BIS-(9-OCTYLAMINO(2-DIMETHYLAMINOETHYL)ACRIDINE-4-CARBOXAMIDE | C44 H54 N8 O2 | 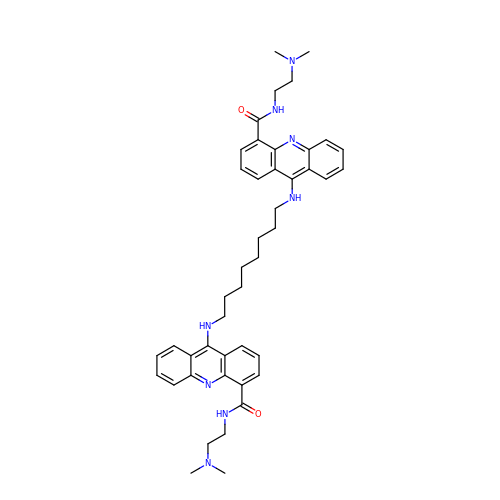UUXARTGDSXDSRM-UHFFFAOYSA-N> GSLDVGNAEV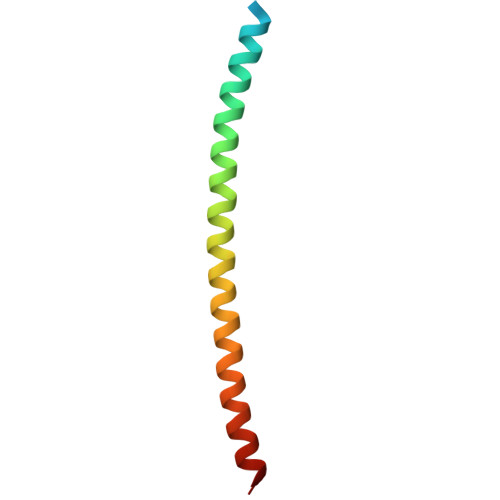KLEEENRSLKADLQKLKDELASTKQKLEKAENQVLAMRKQSEGLTKEYDRLLEEHAKLSAAA> MRGSAHVVILGAGTGGMPAAYEMKEALGSGHEVTLISANDYFQFVPSNPWVGVGWKERDDIAFPIRHYVERKGIHFIAQSAEQIDAEAQNITLADGNTVHYDYLMIATGPKLAFENVPGSDPHEGPVQSICTVDHAERAFAEYQALLREPGPIVIGAMAGASCFGPAYEYAMIVASDLKKRGM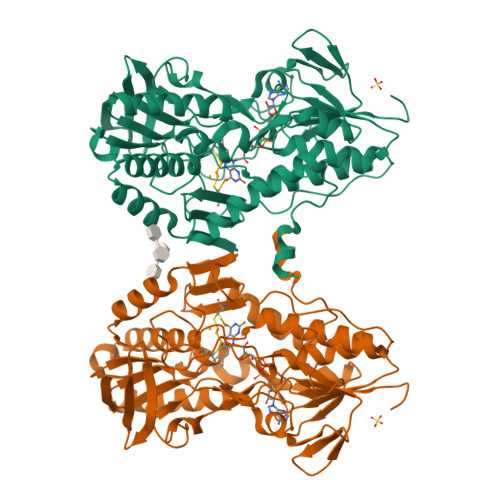RDKIPSFTFITSEPYIGHLGIQGVGDSKGILTKGLKEEGIEAYTNCKVTKVEDNKMYVTQVDEKGETIKEMVLPVKFGMMIPAFKGVPAVAGVEGLCNPGGFVLVDEHQRSKKYANIFAAGIAIAIPPVETTPVPTGAPKTGYMIESMVSAAVHNIKADLEGRKGEQTMGTWNAVCFADMGDRGAAFIALPQLKPRKVDVFAYGRWVHLAKVAFEKYFIRKMKMGVSEPFYEKVLFKMMGITRLKEEDTHRKAS tert-butyl [(2R,6S,12Z,13aS,14aR,16aS)-14a-[(cyclopropylsulfonyl)carbamoyl]-5,16-dioxo-2-{[3-(thiophen-2-yl)quinoxalin-2-yl]oxy}-1,2,3,5,6,7,8,9,10,11,13a,14,14a,15,16,16a-hexadecahydrocyclopropa[e]pyrrolo[1,2-a][1,4]diazacyclopentadecin-6-yl]carbamate 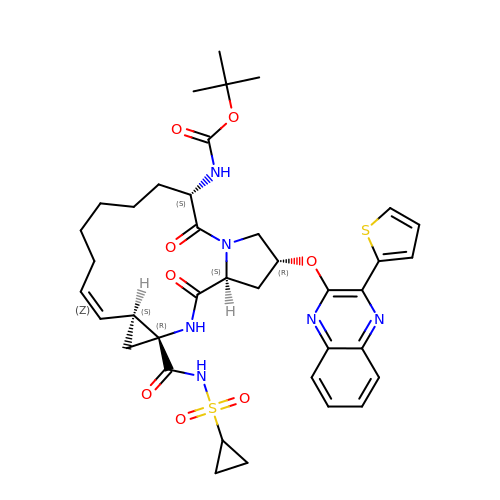| C38 H46 N6 O8 S2 | XPJKLRKWYFSTBR-LZFWIHPHSA-N> MKSVVTTVIAAADAAGRFPSSSDLESVQGSIQRSAARLEAAEKLG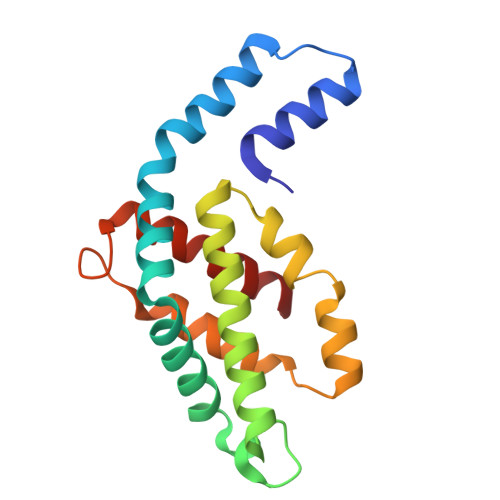ANLDNVAQEAYNACIQKYPYLNNAGEANSNDTYKAKCLRDVKHYMRLIQYCLVVGGTGPLDEWGIAGQREVYRALSLPTAPYVEALSFARNRGCAPRDMSAQALVEYNALLDYAINSLS> GAMGPQEYTLIKLKIHLI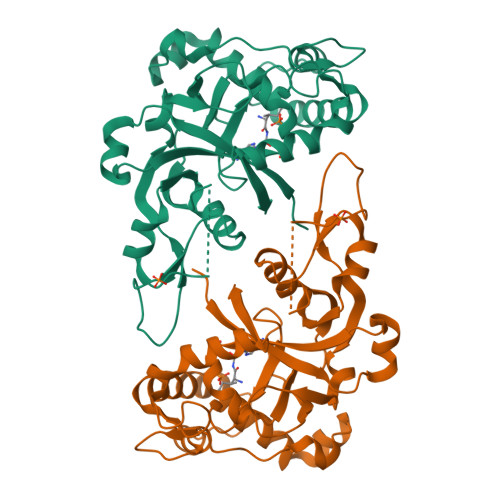PEFLGSIVKGREVFVVCATLRPETMYGQTNCWILPDGEYDLVLAFDQVIPYDAKTSDGVLCKIFDKYEDTMKECNTVYICSERSAYNMAYQGIVPLIHGREQGVSDKLLPRIVSLGKVYGEQLIGTPLSAPMTPYSLIFILPMFSISMEKGTGIVTSVPSDSPDDYAALRDIKTKPLLREKYSIKDEWILDPLEIIEVPGFGFMTAELLCNQYKIQSQNDSAKLKQAKEEIYKKEFYEGILIRGKYSGMKICDAKELIRESLIKDGYALIYLE> VGSLNCIVAVSQNMGIGKNGDLPWPPLRNEFRYFKRMTTTSSVEGKQNLVIMGKKTWFSIPEKFRPLKGRINLVLSRELKEPPQGAHFLSRSLDDALKLTEQPELANKVDM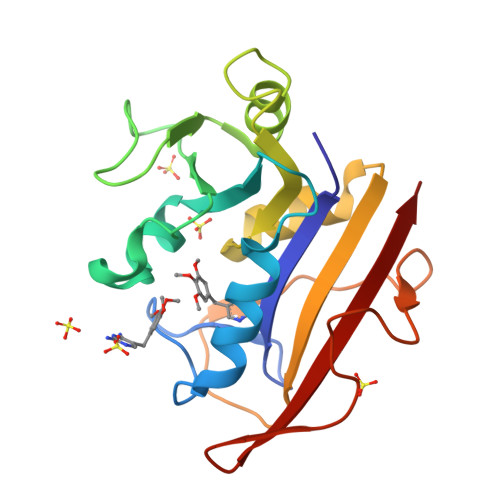VWIVGGSSVYKEAMNHPGHLKLFVTRIMQDFESDTFFPEIDLEKYKLLPEYPGVLSDVQEEKGIKYKFEVYEKND>SLVPRGSGDSGSPGAEYRNWSKPQCQITGFAPFSKDNSIRLSAGGDIWVTREPYVSCSPGKCYQFALGQGTTLNNKHSNGTIHDRIPHRTLLMSELGVPFHLGTKQVCIAWSSSSCHDGKAWLHVCVTGDDRNATASFIYDGMLADSIGSWSQNILRTQESECVCINGTCTVVMTDGSASGRADTRILFIKEGKIVHISPLSGSAQHIEECSCYPRYPDVRCVCRDNWKGSNRPVIDINMADYSIDSSYVCSGLVGDTPRNDDSSSSSNCRDPNNERGNPGVKGWAFDNGNDVWMGRTISEDSRSGYETFRVTDGWTTANSKSQVNRQIIVDNNNWSGYSGIF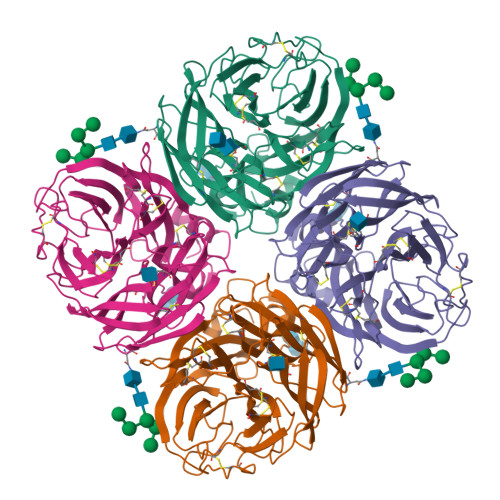SVEGKSCINRCFYVELIRGRPQETRVWWTSNSIVVFCGTSGTYGTGSWPDGANINFMPI[4x]> GSHMVEGFVEPYIRLFEAIPDAETELATFYDADLDTLPPRMFLPSGDLYTPPGPVRLEEIKRKRRVRLVKVSIYRFEHVGLGLAARPYAYAYAWQGDNGILHLYHAPVVLEDVPEVLELDE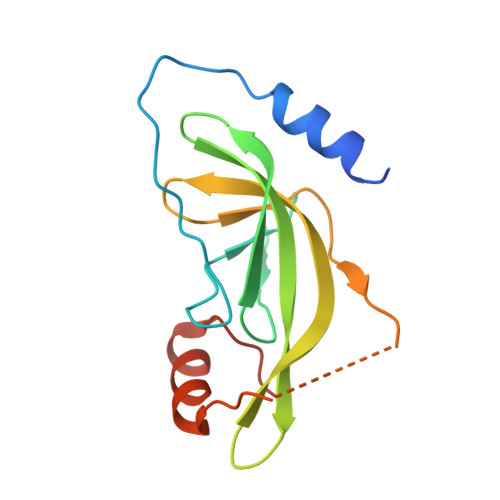VTYNESYVRLMRAMGHVDAFIDL>MGGSHHHHHHGMASMSKRITDSQVLGELGETAIKKIVLETGFLYEQRGRLEAGTDGIIELRDPKSGAPLGKLLGVQVKSTESGQYVRENDNSFEYLLKPDDLKYWRTSNIPVIIVLWRKSDETAYWKDVSDCVRGEERRLKFDKGTDVFDPRSADRIGALTIDRRTPGVFLPPLNKGEDAIINLLRIRLPDEIFISTSPFGSGRDAVPELVKHGNVRFDWVIRKRRFVSFFDPREYGTRAIVDLDQVEAVDTKLIAFNDEQDDLNDTMDLLRRTVERQTATQLSFLRKDRLFHFKAVGVGKSRSYRYMSNVNETSAKVVSAYSSKKKDGWGYVRHHAARLRFERLADEWFLVIDPDFHFTTDGFQPHRYPEALLAGKKRLERNAAVRGQVTMWQHLLVESGKHEVGLFDADKPAPLLQFERLPVIQLSQAVPESSWNRTDPRAKEMEAQDLFEEGGVG[2x];>[2x]MTFKAHVFDEPMLEFGDGGQHCDPRQGLREHGPLQPRSGDVIRVGVIGTDDTVAGFTEFLAETGRGIESGNKQLINLNPDFPGLGNQNPFRCKFEVPDGATVTISRRQVNDITGIGRHDEAVRHAVELISSQLSALVEGSAKPDVIVLALPIPLIEKLVNAKSEGE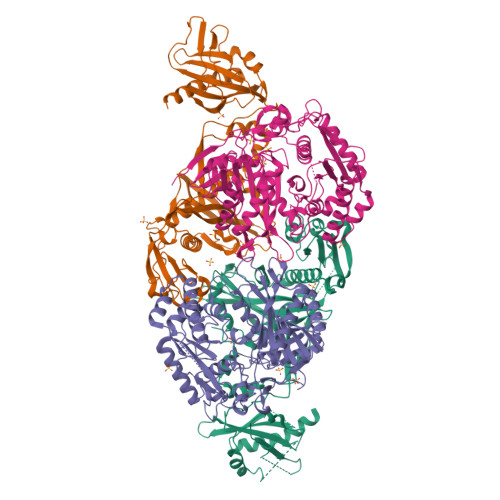DSDDDVDGGDMLNFRDLLKAKTLHLPVPTQIVWPDTWDDAAKIPRKIKRDSNRQTQVKATRAWNLLNALFYKAGKVPWRLLPDQAEYRTSFLGIGFYRDLDGQQLWTSTAQMFDERGRGLILRGARAQTETRGRHPYLTAKDAEDLVVQSIAAYKAHHRHVPARLVVLKTSRFRSEEAEGIDAALGKSGIEMSDLVWVQESSPIAIFRDGNYPVLRGTFVDLDGKGLLYTRGSVPFYGTFPGLRVPRPLLLVPHENSDSTILTLAKDVLALTKVNWNTTQFDQKLPAPIKAAREVGRILKHVEFGTAVSSDFRRYT>MFPEQQKEEFVSVWVRDPRIQKEDFWHSYIDYEICIHTNSMAFTMKTSCVRRRYREFVWLRQRLQSNALLVQLPELPSKNLFFNMNNRQHVDQRRQGLEDFLRKVLQNALLLSDSSLHLFLQSHLNSEDIEACVSGQTKYSVEEAIHKFALMNRRFPEEDE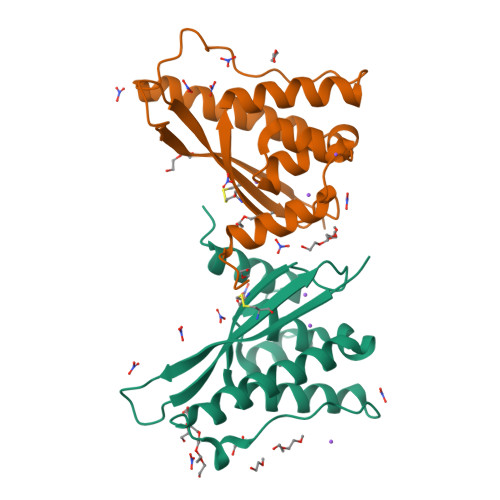EGKKENDIDYDSESSSSGLGHSSDDSSSHGCKVNTAPQESLEHHHHHH[2x]The Picornaviridae family of single-stranded, positive-sense, non-enveloped RNA viruses includes several pathogens of concern such as enterovirus-D68 (EV68). The 3C protease cleaves eight sites within the viral polyprotein, with a preference for a glutamine–glycine (QG) motif at the P1/P1′ positions, a preference distinct from host cysteine proteases. Among strains of EV68, the amino acid sequences of 3C protease and its cleavage sites are highly conserved. We have determined and analyzed three high-resolution inhibitor-bound crystal structures of EV68-3C protease, which revealed possible sites of resistance mutations, a key structural water molecule conserved during ligand binding, and the conformational flexibility of the catalytic histidine H40.

Rupintrivir demonstrated the highest potency with the IC50 value in the single-digit nanomolar range, followed closely by AG7404. Within the active site, rupintrivir and AG7404 exhibited identical hydrogen bonds from P4 to P1′, with one additional hydrogen bond formed between AG7404 and C147 backbone nitrogen. At P2, AG7404 lacked the fluorinated phenylalanine ring of rupintrivir and was unable to pi-stack on the catalytic His40. In this structure, we observed the catalytic His40 in an alternative conformation, where the side chain was rotated furthest away from the substrate-bound position. Between the S2 and S3 pocket, AG7404 contains an aromatic ring incorporated into the peptidomimetic backbone structure that protrudes outside of the substrate envelope. In this region, the mutation of Gly128 into a larger amino acid has the potential to interfere with inhibitor binding and confer resistance. As AG7404 is an analog of rupintrivir, this compound shares many structural similarities and protrudes in the same regions, highlighted at the S4 pocket, where the isoxazole ring forms the same hydrogen bond contact with Asn165. At the S4 pocket, the mutation of Asn165 into a larger residue could preclude binding of the inhibitors, while other mutations could remove the potential for hydrogen bond formation, potentially decreasing inhibitor binding.

> GPGFDFAQAIMKKNTVVARTEKGEFTMLGVHDRVAVIPTHASVGETIYINDVETKVLDACALRDLTDTNLEITIVKLDRNQKFRDIRHFLPRYEDDYNDAVLSVHTSKFPNMYIPVGQVTNYGFLNLGGTPTHRILMYNFPTRAGQCGGVVTTTGKVIGIHVGGNGAQGFAAMLLHSYFTDTQRHHHHHH>[2x]GSEDRDPTQFEERHLKFLQQLGKGNFGSVEMCRYDPLQDNTGEVVAVKKLQHSTEEHLRDFEREIEILKSLQHDNIVKYKGVCYSAGRRNLKLIMEYLPYGSLRDYLQKHKERIDHIKLLQYTSQICKGMEYLGTKRYIHRDLATRNILVENENRVKIGDFGLTKVLPQDKEYYKVKEPGESPIFWYAPESLTESKFSVASDVWSFGVVLYELFTYIEKSKSPPAEFMR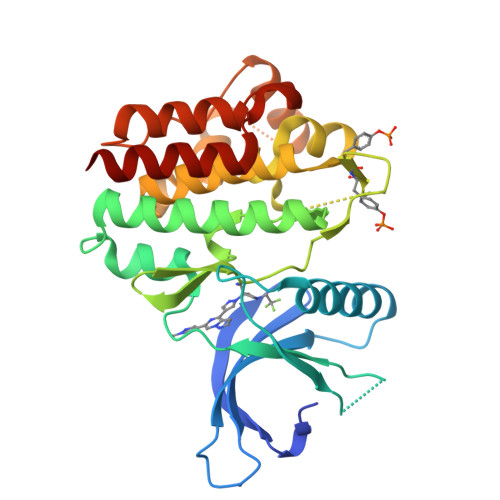MIGNDKQGQSIVTHLIELLKNNGRLPRPDGCPDEIYMIMTECWNNNVNQRPSFRDLALRVDQIRDNMAG> GSSSLQRLEELFRRYKDEREDAILEEGMERFCNDLCVDPTEFRVLLLAWKFQ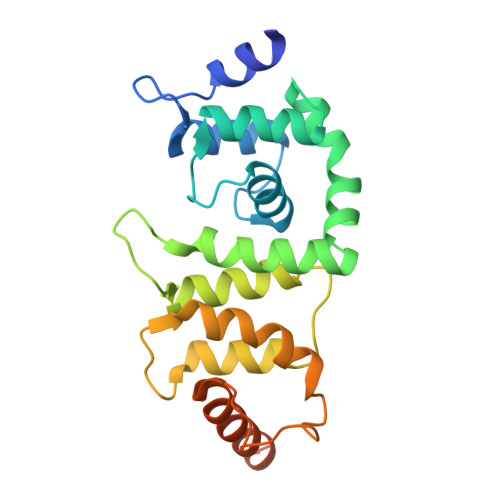AATMCKFTRKEFFDGCKAISADSIDGICARFPSLLTEAKQEDKFKDLYRFTFQFGLDSEEGQRSLHREIAIALWKLVFTQNNPPVLDQWLNFLTENPSGIKGISRDTWNMFLNFTQVIGPDLSNYSEDEAWPSLFDTFVEWEMERRKREGEGRGALSSGPEGLCPEEQT The 12-kDa FK506-binding protein (FKBP12) is a ubiquitously expressed peptidyl-prolyl isomerase with considerable homology between fungal pathogens and is thus a prime candidate for future targeting efforts to generate a panfungal strategy. PPIase proteins all catalyze the cis/trans isomerization of peptide bonds N terminal to proline residues in polypeptide chains. In addition to its role as a PPIase, FKBP12 is a member of the immunophilin family and is the target of the immunosuppressive drugs FK506 and rapamycin. Three extended loops, which have been called the 40s loop (between β2 and β3), the 50s loop (between β3′ and α1), and the 80s loop (between β4 and β5), surround a deep active-site pocket that binds both FK506 and rapamycin.

Three different crystal forms of the apo C. albicans FKBP12, to resolutions of 1.99, 2.3, and 2.4 Å, were obtained. While the C. albicans apo FKBP12 structure is very similar to previously determined FKBP12 structures, an unexpected finding that emerged from analysis of the crystal packing was that despite being obtained under very different crystallization conditions with distinct crystal lattices, all three C. albicans apo FKBP12 structures displayed the same intermolecular interactions between subunits. What is notable about this interaction is that the 80s loop of one subunit docks into the active site of the adjacent subunit and vice versa, suggesting that the loop may act as a substrate. Indeed, Pro104, which is located at the tip of the loop, is inserted most deeply into the pocket and is surrounded by residues that have been implicated, via mutagenesis, to be involved in FKBP PPIase activity. Three residues, in particular, were implicated as important for FKBP12 catalysis and correspond to Val59, Asp41, and Tyr97 in the C. albicans protein. These residues all make direct contacts with Pro104, which rests within an aromatic cleft formed by Tyr30, Phe50, and Trp63. Although most of the contacts that hold the loop in position in the active site are with the central Pro104, additional hydrophobic contacts with Ile102, Pro103, and Ile105 are provided, while Arg100 makes hydrogen bonds with the carbonyl oxygens at the edge of the pocket. Notably, the interface in the C. albicans FKBP12-FKBP12 interaction is minimal (burying 592 Å2 from solvent), which suggests that, like known substrate-enzyme complexes, the proteins form a weak interaction; typical dimer interfaces bury >2,000 Å2 of surface from solvent. Comparison of the C. albicans FKBP12 apo structure with FKBP12-FK506 structures reveals that the 80s loop binds in the same pocket as FK506. Interestingly, unlike the C. albicans apo FKBP12 structures, which were all captured with Pro104 in the cis conformation, in the A. fumigatus structure, Pro90 in one subunit was bound in the cis conformation and Pro90 in the other was bound in the trans state, thus potentially providing a snapshot of self-catalysis.

>[2x]EELPQIEIVQEGDNTTFAKPGDTVTIHYDGKLTNGKEFDSSRKRGKPFTCTVGVGQVIKGWDISLTNNYGKGGANLPKISKGTKAILTIPPNLAYGPRGIPPIIGPNETLVFEVELLGVNGQ>VTEVEQKLQIVHQTLSMLDSHGFENILQEMLQSITLKTGELLGADRTTIFLLDEEKQELWSIVAAGEGDRSLEIRIPADKGIAGEVATFKQVVNIPFDFYHDPRSIFAQKQEKITGYRTYTMLALPLLSEQGRLVAVVQLLNKLKPYSPPDALLAERIDNQGFTSADEQLFQEFAPSIRLILESSRSFYIATQKQRAAAAMMKAVKSLSQSSLDLEDTLKRVMDEAKELMNADRSTLWLIDRDRHELWTKITQDNGSTKELRVPIGKGFAGIVAASGQKLNIPFDLYDHPDSATAKQIDQQNGYRTCSLLCMPVFNGDQELIGVTQLVNKKKTGEFPPYNPETWPIAPECFQASFDRNDEEFMEAFNIQAGVALQNAQL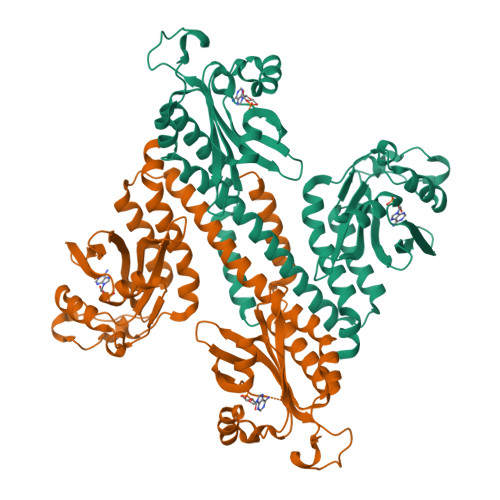FATVKQQEQGSRSHHHHHH[2x]> YIGDFRCIQLVNSNGANVSAPSISTETVEVSQGLGTYYVLDRVYLNATLLLTGYYPVDGSKFRNLALTGTNSVSLSWFQPPYLSQFNDGIFAKVQNLKTSTPSGATAYFPTIVIGSLFGYTSYTVVIEPYNGVIMASVCQYTICQLPYTDCKPNTNGNKLIGFWHTDVKPPICVLKRNFT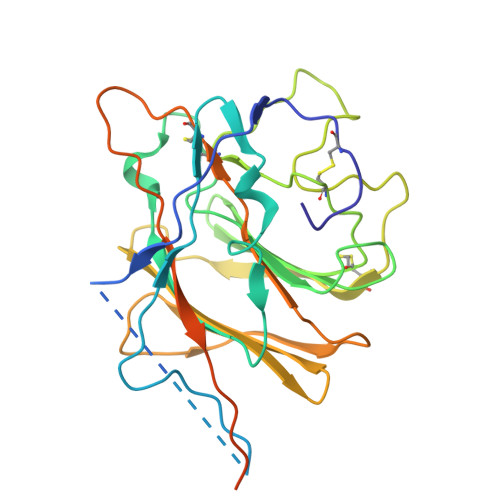LNVNADAFYFHFYQHGGTFYAYYADKPSATTFLFSVYIGDILTQYYVLPFICNPTAGSTFAPRYWVTPLVKRQYLFNFNQKGVITSAVDCASSYTSEIKCKTHHHHHH> GPYGVSQIKAPALHSQGYTGSNVKVAVIDSGIDSSHPALKVAGGASFVPSETNPFQDNNSHGTHVAGTVLAVAPSASLYAVKVLGADGSGQYSWIINGIEWAIANNMDVINMSLGGPSGSAALKAAVDKAVASGVVVVAAAGNEGTSGSSSTVGYPGKYPSVIAVGAVDS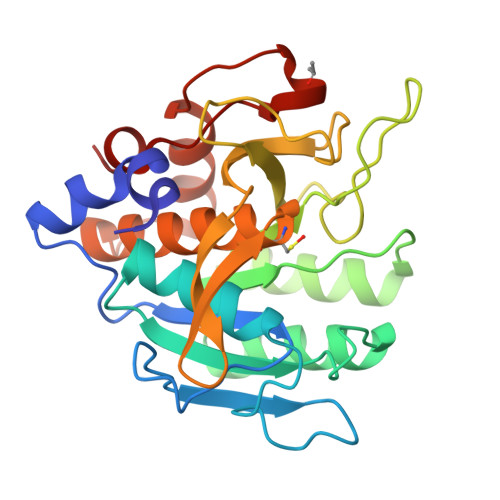SNQRASFSSVGPELDVMAPGVSIWSTLPGNKYGAKSGTCMASPHVAGAAALILSKHPNWTNTQVRSSLENTTTKLGDSFYYGKGLINVEAAAQ N-({3-[5-hydroxy-3-methyl-4-(1H-pyrrolo[3,2-c]pyridin-2-yl)-1H-pyrazol-1-yl]phenyl}methyl)-N'-phenylurea | C25 H22 N6 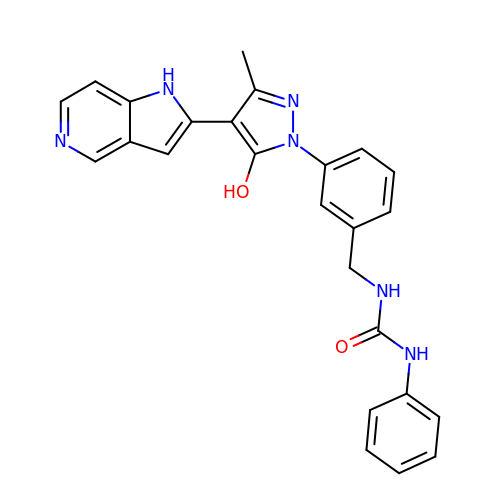O2 | NMKKTNKAENJFOY-UHFFFAOYSA-N> SSKEVAELKKQVESAELKNQRLKEVFQTKIQEFRKACYTLTGYQIDITTENQYRLTSLYAEHPGDCLIFKATSPSGSKMQLLETEFSHTVGELIEVHLRRQDSIPAFLSSLTLE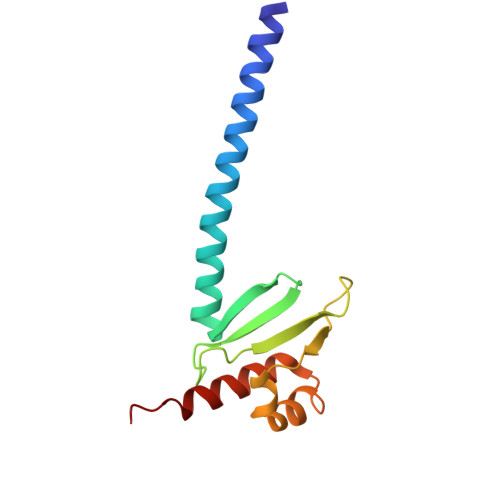LFSRQTVA> MLIAIE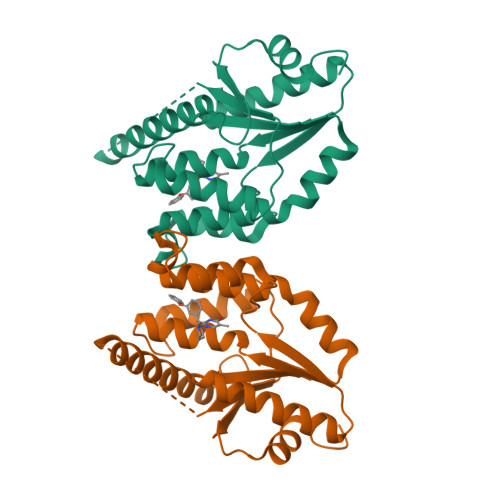GVDGAGKRTLVEKLSGAFRAAGRSVATLAFPRYGQSVAADIAAEALHGEHGDLASSVYAMATLFALDRAGAVHTIQGLCRGYDVVILDRYVASNAAYSAARLHENAAGKAAAWVQRIEFARLGLPKPDWQVLLAVSAELAGERSRGRAQRDPGRARDNYERDAELQQRTGAVYAELAAQGWGGRWLVVGADVDPGRLAATLAPPDVPS>GIVNVPNPNNTKFQELARFAIQDYNKKQNAHLEFVENLNVKEQVVAGIMYY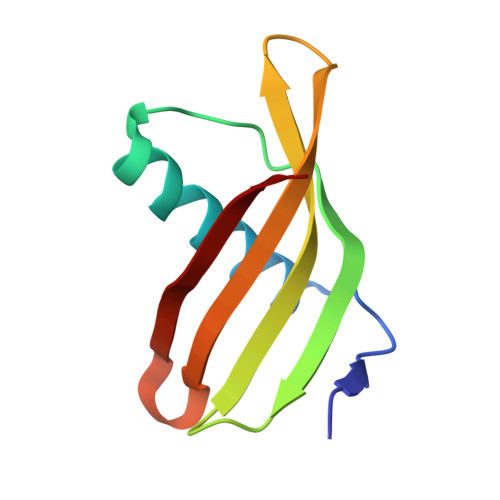ITLAATDDAGKKKIYKAKIWVKEWEDFKKVVEFKLV[14x]>[12x]GSMREE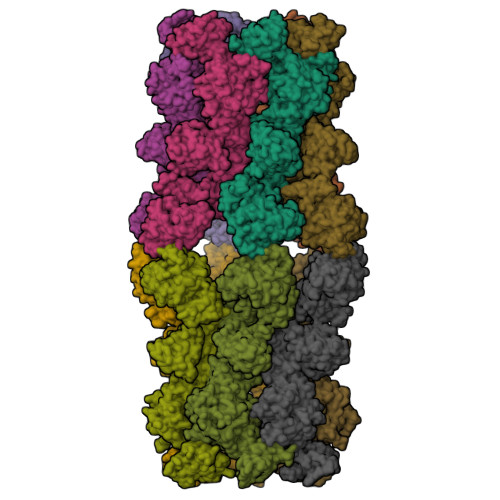SWEEHDTIQLTAQRKYLAEVQALETLLARELSVFLTEPGSKKTNIINRITGKTYALPSTELLRFYEHLEQCRKQGALMYFLERQGTYSGLMLDYDLKLNTNAAPSLESSVLSRLCHRIFVHIKNSSVLPEGSHKIHFFFTLKPEAVQGKYGFHVLIPGLKMAASTKKSIIASLQHDATVQKILHEQGVANPESCLDPHSASVPSLLYGSSKLNHRPYQLKTGFELVFDSSDPDYIPIHQIKNIESYNLVSELSLTNEQGSLVRPVYCAADIAAEKEEEIPADDHSLSILMLHDPEARYLHKILNLLPPEYYVEYPLWSNVVFALANTSANYRPLAEWFSQKCPEKWNTGGKEKLEKLWNDASRHTEKKITKRSIMYWAHKHAPQQYKEIVEQGYFSILAEYVYSYNGTLEHYMIAKVIYAMMGNKFVVDVDSNGKYVWFEFVLPGQPMNQGEIWKWRKEVNPDELHIYISENFSRVMDRITEHIKYHLSQPHETNILNYYKKLLKAFERSKSKIFNDSFKKGVIRQAEFLFRQRSFIQTLDTNPYLLGVGNGVLSIETIPAKLINHFHEHPIHQYTHICYEPFNPENPWTKLLLNALQDIIPELDARLWIMFYLSTAIFRGLKEALMLLWLGGGCNGKTFLMRLVAMVLGDHYASKLNISLLTSYRETAEKPNSAFMRLKGRGYGYFEETNKSEILNTSRLKEMVNPGDVTARELNQKQESFQMTATMVAASNYNFIIDTTDHGTWRRLRHYRSKVKFCHNPDPNNSYEKKEDPRFIHEYIMDPNCQNAFFSILVYFWEKLQKEYNGQIKKVFCPTIESETEAYRKSQDTLHRFITERVVESPSAETVYNLSEVVTAYAEWYNANINVKRHIALELSQELENSVLEKYLQWSPNKTRILKGCRILHKFETLQPGESYIGVSSTGTLLNTPICEPKNKWWEWSPNPSAPPEKEASAPTP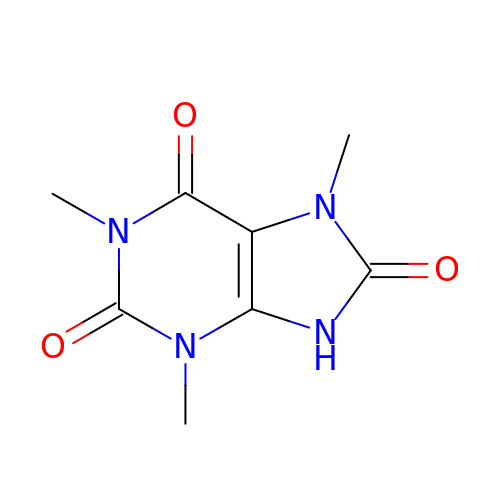1,3,7-trimethyl-9H-purine-2,6,8-trione | C8 H10 N4 O3 | BYXCFUMGEBZDDI-UHFFFAOYSA-N> MADTRIGVTIYKYDDCFMSVVRKAIEQDAKAAPDVQLLMNDSQNDQSKQNDQIDVLLAKGVKALAINLVDPAAAGTVIEKARGQNVPVVFFNKEPSRKALDSYDKAYYVGTDSKESGIIQGDLIAKHWAANQGWDLNKDGQIQFVLLK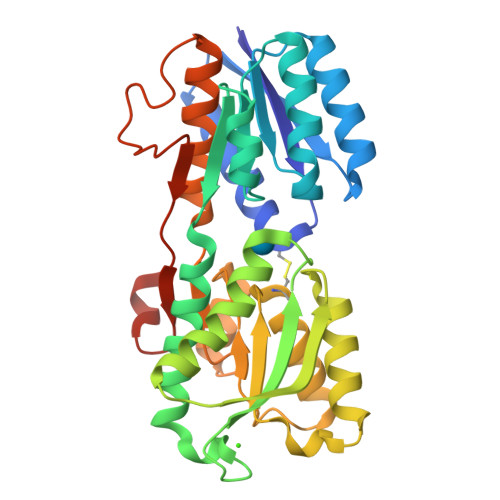GEPGHPDAEARTTYVIKELNDKGIKTEQLQLDTAMWDTAQAKDKMDAWLSGPNANKIEVVIANNDCMAMGAVEALKAHNKSSIPVFGVDALPEALALVKSGALAGTVLNDANNQAKATFDLAKNLADGKGAADGTNWKIDNKVVRVPYVGVDKDNLAEFSKKGSHHHHHH> MHPGFFTSIGQMTDLIHTEKDLVTSLKDYIKAEEDKLEQIKKWAEKLDRLTSTATKDPEGFVGHPVNAFKLMKRLNTEWS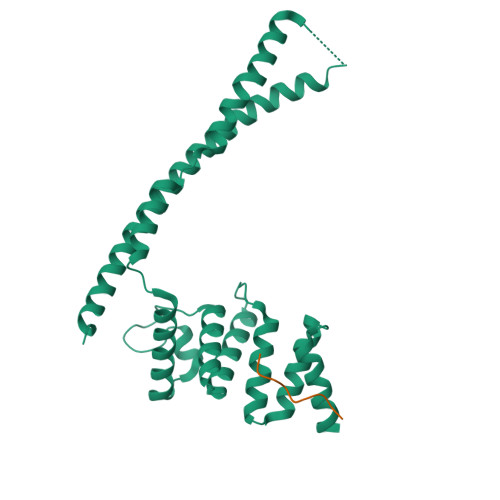ELENLVLKDMSDGFISNLTIQRQYFPNDEDQVGAAKALLRLQDTYNLDTDTISKGNLPGVKHKSFLTAEDCFELGKVAYTEADYYHTELWMEQALRQLDEGEISTIDKVSVLDYLSYAVYQQGDLDKALLLTKKLLELDPEHQRANGNLKYFEYIMAKE;> PPPPPPPPP>AYTT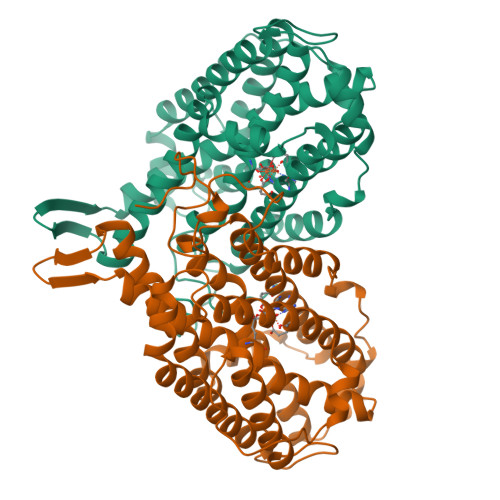FSQTKNDQLKEPMFFGQPVNVARYDQQKYDIFEKLIEKQLSFFWRPEEVDVSRDRIDYQALPEHEKHIFISNLKYQTLLDSIQGRSPNVALLPLISIPELETWVETWAFSETIHSRSYTHIIRNIVNDPSVVFDDIVTNEQIQKRAEGISSYYDELIEMTSYWHLLGEGTHTVNGKTVTVSLRELKKKLYLCLMSVNALEAIRFYVSFACSFAFAERELMEGNAKIIRLIARDEALHLTGTQHMLNLLRSGADDPEMAEIAEECKQECYDLFVQAAQQEKDWADYLFRDGSMIGLNKDILCQYVEYITNIRMQAVGLDLPFQTRSNPIPWINTWLV[2x]In this study we show that IbpS, a protein secreted by D. dadantii, can bind Fe3+ and Cu2+. We demonstrate that exogenously added IbpS reduces the toxicity of H2O2, probably by preventing the Fenton reaction. Our work establishes that members of the Ibp family exhibit the same fold as SBP proteins albeit with significant modifications making of IbpS structure a prototype for this family. The reduced pathogenicities of D. dadantii ibpS and Botrytis cinerea ibp mutants reveal the importance of this conserved protein in the infectious process deployed by necrotrophic microbes probably because of their impaired capacity to detoxify ROS produced during infection.

In the case of iron, the protein was co-crystallized with FeCl3 and the structure of iron bound IbpS was solved at a resolution of 1.8 Å. The protein crystalized in a different crystal form with the P1 space group and four molecules per asymmetric unit. All four molecules were bound to a single-iron atom at the same binding site. The structures of IbpS and Fe-IbpS were nearly identical and no important structural modification was observed. As suspected from our previous analysis, the metal did not bind at the canonical SBP cluster D protein substrate-binding pocket. Instead, the iron atom was located near the dimer interface, at the entry of tunnel identified previously. The metal sits in a cavity formed by residues S86, K87, Q110, T111, M334, and a triple aspartate motif of the α5-β8 loop (D191, D192, D193) and containing a dense network of water molecules. Nevertheless, the conservation of the residues involved in iron-binding in IbpS strongly suggests that the binding site identified here accomplishes a common, essential function in all members of this family.

>MQYTGKYLKKTALMLTMMAGLSAGQSQATVAPDTRSLDEIYQSALKEGGTVTVYAGGDVQSQQAGFKQAFENRFPGIKLNVIVDYSKYHDARIDNQLATDTLIPDVVQLQTVQDFPRWKKQGVLLNYKPVGWDKVYPEFRDADGAWIGAYVIAFSNLVNTQLLNEKSWPREANDYLRPDLKGNLILAYPNDDDAVLFWYKQIVDKYGWEFVEKLQEQDPVYVRGTNVPGAQITTGKYSATFTSSGALVPAAGSVTRFVLPKTDPFVSWAQRAAIFKQAKHPESAKLYLSWLLDPQTQTQVSRMWSVRTDVAPPAGYKHIWEYSNTRPQAFADFMSDRGAVERFRAQMSLYVGEAKGDPTPGWLGLHPEVPLAN[4x]> AFDGTWKVDRNENYEKFMEKMGINVVKRKLGAHDNLKLTITQEGNKFTVKESSNFRNIDVVFEL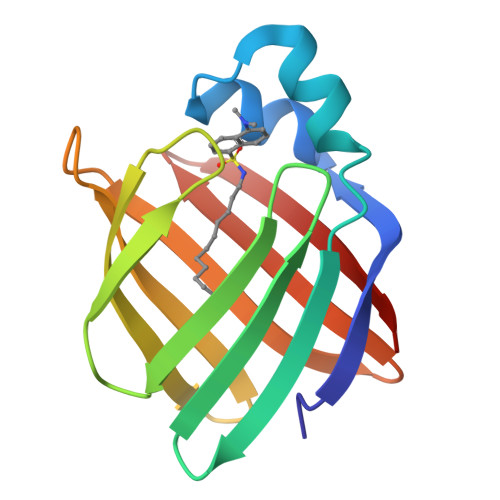GVDFAYSLADGTELTGTWTMEGNKLVGKFKRVDNGKELIAVREISGNELIQTYTYEGVEAKRIFKKE1-[4-[4-[2-[[4-chloranyl-3-(diethylsulfamoyl)phenyl]amino]pyrimidin-4-yl]pyridin-2-yl]phenyl]-3-methyl-urea 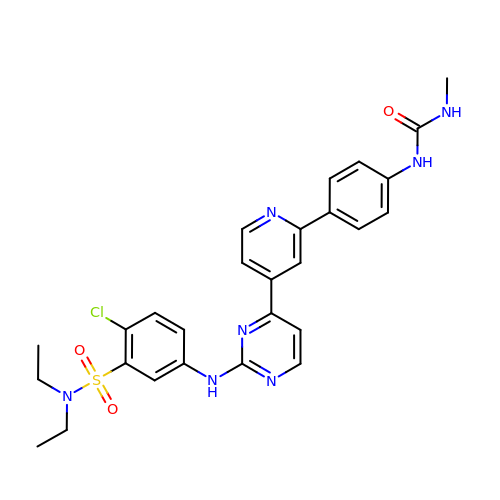| C27 H28 Cl N7 O3 S | RZFJBSIAXYEPBX-UHFFFAOYSA-N R-Talinolol 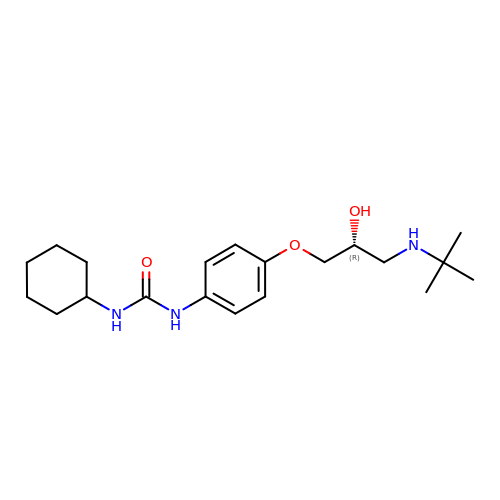| C20 H33 N3 O3 | MXFWWQICDIZSOA-QGZVFWFLSA-N> GSHMASLRHSMDPPTFTFNFNNEPWVRGRHETYLCYEVERMHNDTWVLLNQRRGFLCNQAPHKHGFLEGRHAELCFLDVIPFWKLDLDQDYRVTCFTSWSPCFSCAQEMAKFISKNKHVSLCIFTARIYDDQGRCQEGLRTLAEAGAKISIMTYSEFKHCWDTFVDHQGCPFQPWDGL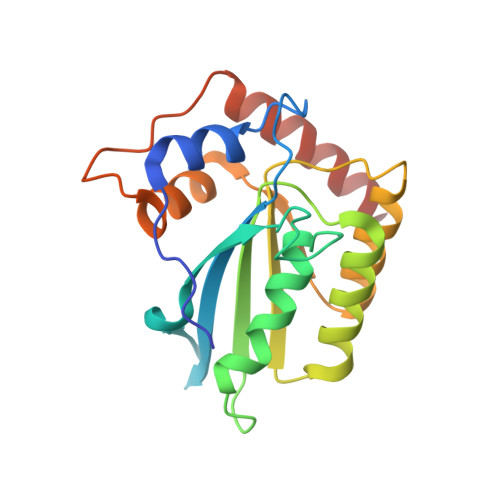DEHSQALSGRLRAILQNQEN>VVGGVVX[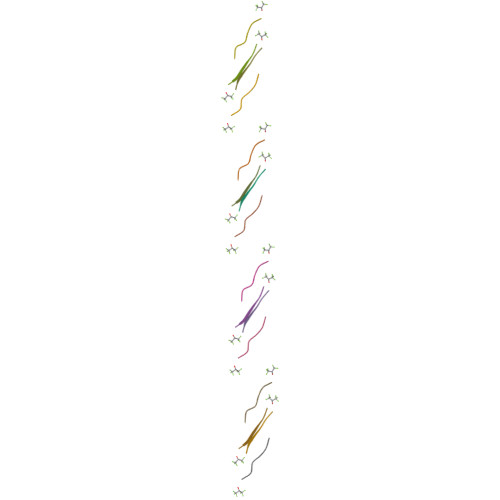4x]All BoNTs are naturally co-expressed with a protective partner protein (NTNH) with which they form a 300 kDa complex, to resist acidic and proteolytic attack from the digestive tract. We have previously identified a new botulinum neurotoxin serotype, BoNT/X, that has unique and therapeutically attractive properties. We present the cryo-EM structure of the BoNT/X-NTNH/X complex and the crystal structure of the isolated NTNH protein. BoNTs are 150 kDa proteins and consist of three domains: the 50 kDa catalytically active light chain (LC) and the 100 kDa heavy chain that is further divided into the translocation domain (HN) and the receptor-binding domain (HC).

We have determined the cryo-EM structure of the M-PTC/X complex comprising the BoNT/X R360A/Y363F inactive mutant holotoxin and its non-toxic interaction partner NTNH/X at a nominal resolution of 3.1 Å (using the gold-standard FSC criterion of 0.143), obtained from 432,063 particles selected from a total of 5408 recorded movies from two datasets in similar data acquisition settings, described in the “Materials and methods” section. BoNT/X and NTNH/X share a similar fold and their overall domain arrangement and molecular architecture is similar to other toxin serotypes. Similarly to the known M-PTC structures of the A and E serotypes, BoNT/X and NTNH/X form an interlocked complex that buries a large solvent-accessible area of 4778 Å2, which is significantly larger compared to BoNT/A-NTNH/A (3664 Å2) and BoNT/E-NTNH/E (3459 Å2). The main domains that are involved in this interaction are the receptor-binding domain in BoNT/X (HC/X) and the analogous domain in NTNH/X (nHC/X), together with the translocation domain and its analog (HN/X and nHN/X). LC and nLC are situated in both extremities of the complex, facing opposite directions from the interface, and are mostly solvent-exposed. Our cryo-EM map indicates that C423-C467 is the most likely natural disulfide bridge. A cluster of solvent-accessible acidic and basic residues can be found on the interface between HCN/X and nHN/X, namely D998, K1000, K1046, E1048, E1049, K1050, D1051, K1013, and D1018 in BoNT/X; and K636, E787, E789, and E793 in NTNH/X. The location of this pH-sensing cluster corresponds to a similar cluster in BoNT/A-NTNH/A, which has been demonstrated to drive the pH-mediated disassembly of the M-PTC/A13. The charge of these residues will depend on the environmental pH, which was pH 5.5 in the buffer utilized for the cryo-EM experiments. Although there is no particular sequence conservation for that region, BoNT/X in the M-PTC structure also presents a flexible linker followed by a small helical conformation leading to HC (residues 876–895). The BoNT/X-NTNH/X complex structure also provides structural information on the receptor-binding domain of BoNT/X, which revealed an unusual array of surface-accessible hydrophobic patches despite presenting the same overall fold as other BoNTs.

> MDINDKLSIDSPIDNKNIIEFITFRTDTSGIQKKIKAYQIAKHIWVVPERYYAEPLNISDEYKIDGGIYNENYLTTDKERQEYLDAICILFKRINNVIEGKKLLSLLSSASPFPFKDDTNKYLLKEALLYVNEENFEFKFFTSNIILFGPGTNISKNQVLPLNGDDATSGVGSVSEICYNPFFTKKFGEYSLDPVIGLIECLLKSLYNLYGIKVSDDIKIPYKLQRALNTDKYSYINLEEALIFGGNDYKIFTEKPYWLSNDYFLKSLNTFEENKAKYEKDLKNDPNLNNELNQYLQQKYSFSISKIWSLNLTAFADIFNINIPTSFLASITFWDRSQYYKINYPNDYNIDGFVNGQWNTNLKNIEKDNNFIIFDKPKQIITYINDIFNLRYTSNLYEDNLDIESNNYYLNFMFEYDKGNNFTINQYKALLDTLDNDFIDSLPPIQGMNAQNKLTSLPIISKGTDTENINSELLLPIHYLKSQTYNLDMYSSIKFTTNIYEVVSEKNSELVYTFLPHINEIMENYSINNTIKTEEEFYNWMENLFINYSIDILEKRNSIIPGITAVLPWIGKALNILNTNNDFEEELQLSGIKGLIKEYENFIIPDMIVPDIPLDNMPRTYDDIDKKLSEIYTKNKFLFLKGYYFIVQEWWTTYYIQFIELKYLCSGAINKQQQLLITVLEKQLFYFTNNGLFPFDAMERMINEFNRSIDIFSRISQQALNNVDIFINECALFIFNNEVYPLFLNNVENNINKANDNVLNYINKATSLTEEQIKELTVKYTFSSIAEVEFFNESYFKKITNMDIKNILTNIKNINNLILSGSQINDDITIFDESGNNLNIKFDPSIRIVDGHTNVAFKLDKSSQYINIPTENINFSFMESFSIDFWLKILDSTESTTLLNCIEDDIGWKLSIQNNNLLWEMKDNLGNNFTSLFTFNINNIWHNITLSIDRLTNTFNCFLDGKLINTDNISNIFSLETNTPIEIQSDNGAILLEAFSILNYPLQQQEVLNRYREAFSNNYTRNYYGDILKYNENYQLYNKTSPDKEVKKVFTNDKDYIAIEYNQNTNNPTFFSLIQKEQSKIYVEENDEVYICVQGDPLNYITIDNNQAVLTKDINLATSFKLKTNLNKPNSLIFSENSQALRLSNRLNDENYILLDLVSKLDDEPLNIFYWEFI;> MKLEINKFNYNDPIDGINVITMRPPRHSDKINKGKGPFKAFQVIKNIWIVPERYNFTNNTNDLNIPSEPIMEADAIYNPNYLNTPSEKDEFLQGVIKVLERIKSKPEGEKLLELISSSIPLPLVSNGALTLSDNETIAYQENNNIVSNLQANLVIYGPGPDIANNATYGLYSTPISNGEGTLSEVSFSPFYLKPFDESYGNYRSLVNIVNKFVKREFAPDPASTLMHELVHVTHNLYGISNRNFYYNFDTGKIETSRQQNSLIFEELLTFGGIDSKAISSLIIKKIIETAKNNYTTLISERLNTVTVENDLLKYIKNKIPVQGRLGNFKLDTAEFEKKLNTILFVLNESNLAQRFSILVAKHFLKERPIDPIYVNILDDNSYSTLEGFNISSQGSNDFQGQLLESSYFEKIESNALRAFIKICPRNGLLYNAIYRNSKNYLNNIDLEDKKTTSKTNVSYPCSLLNGCIEVENKDLFLISNKDSLNDINLSEEKIKPETTVFFKDKLPPQDITLSNYDFTEANSIPSISQQNILERNEELYEPIRNSLFEIKTIYVDKLTTFHFLEAQNIDESIDSSKIRVELTDSVDEALSNPNKVYSPFKNMSNTINSIETGITSTYIFYQWLRSIVKDFSDETGKIDVIDKSSDTLAIVPYIGPLLNIGNDIRHGDFVGAIELAGITALLEYVPEFTIPILVGLEVIGGELAREQVEAIVNNALDKRDQKWAEVYNITKAQWWGTIHLQINTRLAHTYKALSRQANAIKMNMEFQLANYKGNIDDKAKIKNAISETEILLNKSVEQAMKNTEKFMIKLSNSYLTKEMIPKVQDNLKNFDLETKKTLDKFIKEKEDILGTNLSSSLRRKVSIRLNKNIAFDINDIPFSEFDDLINQYKNEIEDYEVLNLGAEDGKIKDLSGTTSDINIGSDIELADGRENKAIKIKGSENSTIKIAMNKYLRFSATDNFSISFWIKHPKPTNLLNNGIEYTLVENFNQRGWKISIQDSKLIWYLRDHNNSIKIVTPDYIAFNGWNLITITNNRSKGSIVYVNGSKIEEKDISSIWNTEVDDPIIFRLKNNRDTQAFTLLDQFSIYRKELNQNEVVKLYNYYFNSNYIRDIWGNPLQYNKKYYLQTQDKPGKGLIREYWSSFGYDYVILSDSKTITFPNNIRYGALYNGSKVLIKNSKKLDGLVRNKDFIQLEIDGYNMGISADRFNEDTNYIGTTYGTTHDLTTDFEIIQRQEKYRNYCQLKTPYNIFHKSGLMSTETSKPTFHDYRDWVYSSAWYFQNYENLNLRKHTKTNWYFIPKDEGWDED>MGAEIPKEMLRAQTNVILLNVLKQGDNYVYGII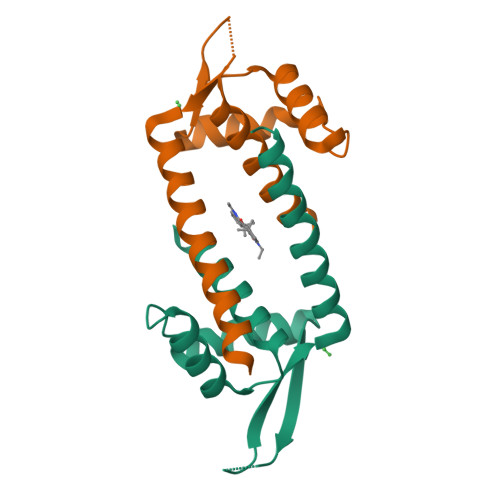KQVKEASNGEMELNEATLYTIFDRLEQDGIISSYAGDESQGGRRKYYRLTEIGHENMRLAFESWSRVDKIIENLEANKKSEAIKSRGGSGGASHPQFEK[4x]7-[6-(dimethylamino)pyridin-3-yl]-~{N}-[[(3~{S})-piperidin-3-yl]methyl]pyrido[3,4-b]pyrazin-5-amine 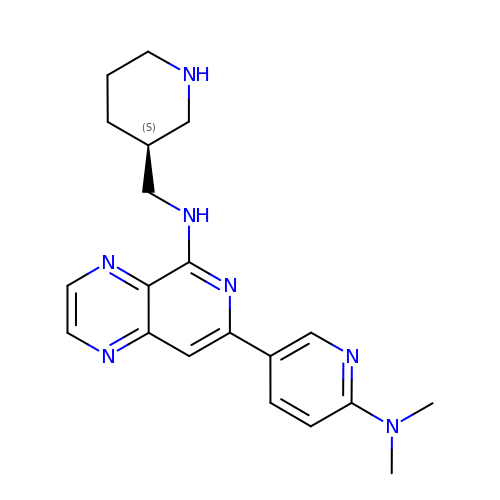| C20 H25 N7 | CLKZDZYGBHNPSM-AWEZNQCLSA-N> EYAPLTVSVIVQDEGIDAIPVKVLNCDTISQVKEKIIDQVYRTQPCSCWPKPDSVVLEW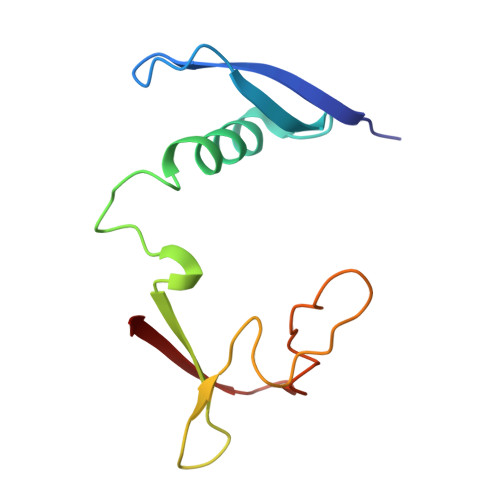RPGSTAQILSDLDLTSQREGRWKRINTLMHYNVRDGATLILSKV FhCyLS-2 from F. hepatica is an unusual member of the superfamily, where our sequence and 3D structure analyses in this study revealed that it combines characteristics of both families. The protein architecture demonstrates its relationship to stefins, but FhCyLS-2 also contains the secretion signal peptide and disulfide bridges typical of true cystatins. We determined that FhCyLS-2 is a broad specificity inhibitor of cysteine cathepsins from both the host and F. hepatica, suggesting a dual role in the regulation of exogenous and endogenous proteolysis. Based on phylogenetic analysis that identified several FhCyLS-2 homologues in liver/intestinal foodborne flukes, we propose a new group within the cystatin superfamily called cystatin-like stefins.

The crystal structure of recombinant FhCyLS-2 was determined by single isomorphous replacement and refined using native data to 1.60 Å resolution. FhCyLS-2 crystallized in an orthorhombic space group C2221 with one molecule in the asymmetric unit and a solvent content of 48.3%. The final model of FhCyLS-2 contained 93 residues (Val4–Thr96). The molecule adopted a typical fold of classical stefins like the human homologues stefins A and B. In contrast to stefins A and B, the intact C-terminal strand β4 was split into two smaller β-strands in FhCyLS-2. Importantly, FhCyLS-2 incorporated two disulfide bridges into the disulfide-free scaffold of stefins. They were located in loops at the edge of the β-sheet and indicated as D1 (Cys39-Cys66) and D2 (Cys69-Cys95). While the positions of the C-terminal disulfides (D2 and D4) were similar, the upstream disulfides formed an interloop bridge (D1) in FhCyLS-2 but an intraloop bridge (D3) in the cystatins D and F.

> VGGYTEPRSVTPEERSVFQPMILSKLLTAGSVVSSCELELLQVSTQVVAGTNYKFKVSGGATCPGCWEVVVFVPLYSSKSATSVGTPTRVSCT> MDNYIYSIAHQLYEMYLQDEDAFHSKRDYPHKKVFTELQKLRKIFFPDFFMKHQKITESHIASELTKLVDYIKDSVTAYNDELFAHQCVMAILEKLPSIKRTLKTDLIAAYAGDPAAPGLSLIIRCYPGFQAVIVYRIAHVLYECGERYYCREMMESVHS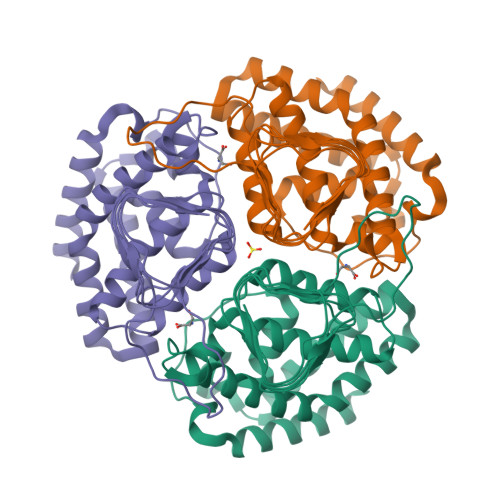YTSIDIHPGASIKGHFFIDHGVGVVIGETAIIGEWCRIYQSVTLGAMHFQEEGGVIKRGTKRHPTVGDYVTIGTGAKVLGNIIVGSHVRIGANCWIDRDVDSNQTVYISEHPTHFVKPCTTKGMKNDTEIIAIIPSSPLANSPSILEHHHHHH> GPLGSEEDILARVDLETTRAIAKQMFSSGTVVEVSSDEEGFQGCWFAAKVVEPVGEDKFLVEYRDLREKDGIEPLKEETDFLHIRPPPPRDEDIDFAVGDKINAFYNDGWWVGVVIDGMKHGTVGIYFRQSQEKMRFGRQGLRLHKDWVDGTWQLPLK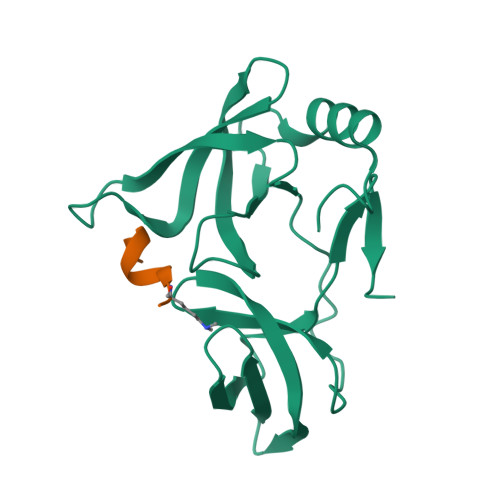GG;> ARTKQTARKS> MLRRGAKELVQLLRTPVKQ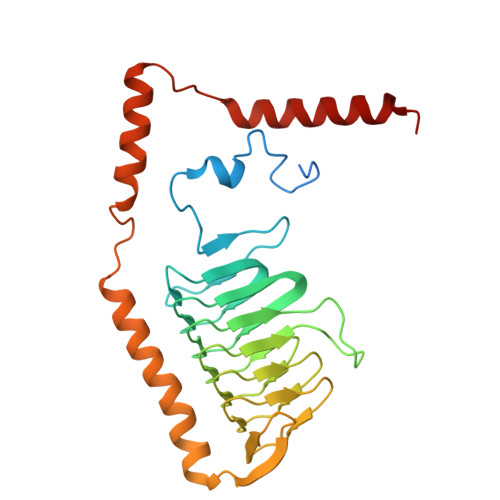GAQLQYVATRNVNFYDAPNGPAVEQVKIEDEWYNRQRTEFNILNKQPSKADDVFIAPNAVVCGDVDLYQKVSIFFGAVVRGDLNTIRIGENSTILDKAVVHAASTSPTGLNAATIIGSNVTVEPHAVLRSCRIGDNCIVGARSVVCEGAIMHPESVLAPGSVLAPGRQIPSGELWAGSPAKFVRKLTYYETSNVIRESAEHYYDIATGFRNETFDHGSAWRDAEAYRQKLVDYKEYNWVNYREQKYVMRLQRDAAELEKLL> MSSKPTDRGQQYKDGKFTQPFSLVNQPDAVGAPINAGDFAEQINHIRNSSPRLYGNQSNVYNAVQEWLRAGGDTRNMRQFGIDAWQMEGADNYGNVQFTGYYTPVIQARHTRQGEFQYPIYRMPPKRGRLSSRAEIYAGALSDKYILAYSNSLMDNFIMDVQGSGYIDFGDGSPLNFFSYAGKNGHAYRS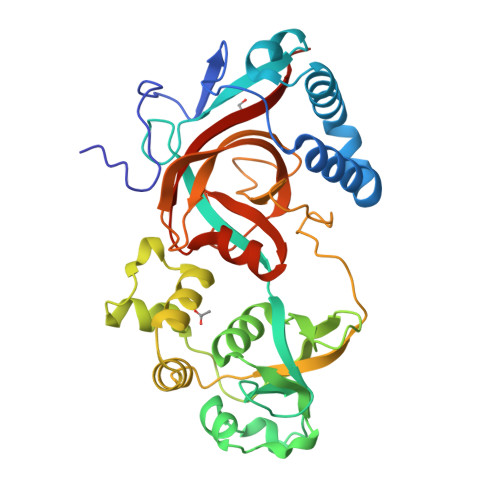IGKVLIDRGEVKKEDMSMQAIRHWGETHSEAEVRELLEQNPSFVFFKPQSFAPVKGASAVPLVGRASVASDRSIIPPGTTLLAEVPLLDNNGKFNGQYELRLMVALDVGGAIKGQHFDIYQGIGPEAGHRAGWYNHYGRVWVLKTAPGAGNVFSG Here, we show that a tyrosine phosphoregulatory system controls the biosynthesis and abundance of Vibrio exopolysaccharide (VPS), an essential biofilm component of the pathogen Vibrio cholerae. The phosphorylation state of the tyrosine autokinase VpsO, mediated by the tyrosine phosphatase VpsU, directly modulates VPS production and also affects the kinase’s own degradation, to regulate VPS production. We found that VpsO and VpsU have respective kinase and phosphatase functions, and we have determined crystal structures of VpsU and the VpsO catalytic domain. We found that the VpsU tyrosine phosphatase controls VPS production through regulation of the VpsO phosphorylation state. Together, our data suggest that the phosphorylation state of the C-terminal tail of VpsO, modulated by autokinase and VpsU phosphatase activity, regulates the functional state of VpsO to control VPS production and biofilm formation in V. cholerae.

VpsU is a 166-amino-acid cytoplasmic protein containing the hallmark C(X)5R motif of the low-molecular-weight phosphotyrosine phosphatase (LMW-PTP) superfamily. We next determined the crystal structure of VpsU at 2.2-Å resolution. The two molecules in the asymmetric unit form a domain-swapped dimer. The overall fold of each monomer is similar to that of other prokaryotic and eukaryotic LMW-PTPs. It contains a central four-stranded parallel β-sheet flanked by two α-helices on one side and three α-helices on the other side. VpsU contains the same complement of active site residues as other prokaryotic LMW-PTPs including the nucleophilic cysteine (C12) and the tyrosine (Y127) that stacks with the substrate phosphotyrosine. In the crystal, domain swapping in the dimer occurs through exchange of the C-terminal α-helix (α5). Although size-exclusion chromatography data were consistent with dimerization, we cannot be sure that domain swapping also occurs in solution. In a steady-state kinetic analysis of the wild-type activity, we measured the KM to be 0.9 ± 0.1 mM and the kcat to be 1.4 ± 0.1 min-1. These findings suggest that VpsU has phosphotyrosine phosphatase activity and that cysteine 12 is necessary for catalytic activity. Collectively, these results show that VpsU dephosphorylates VpsO in vitro.

>[2x]MKVKGLSVLVVCTGNLCRSPMAEIILRDKIRQKRLNIQVRSAGTLKTGKTMPDDKALQALQDYGYHPMVNPVQQVTQQDFIEHDFIYAMDRTNLADLLDICPAEHKNKLALFLSKANRQEKEVPDPYRRSSEFFQRTALLIESGAVALVDSWQEQGINACNENLSQ> SNAHITLDPDTANPWLILSEDRRQVRLGDTQQSIPGNEERFDSYPMVLGAQHFHSGKHYWEVDVTGKEAWDLGVCRDSVRRKGHFLLSSKSGFWTIWL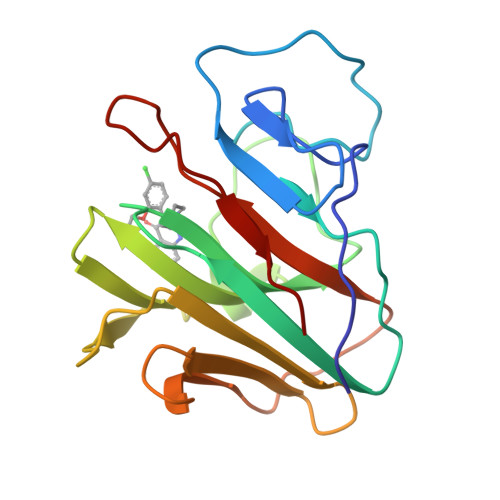WNKQKYEAGTYPQTPLHLQVPPCQVGIFLDYEAGMVSFYNITDHGSLIYSFSECAFTGPLRPFFSPGFNDGGKNTAPLTLCPL>[2x]MAAAAAAEVSVDEKLDKLRAEVAKLDQISENEKAGFISLVSRYLSGEAEQIEWSKIQTPTDEVVVPYDTLASPPEDLEETKKLLDKLVVLKLNGGLGTTMGCTGPKSVIEVRNGFTFLDLIVIQIESLNKKYGCSVPLLLMNSFNTHDDTQKIVEKYSNSNIEIHTFNQSQYPRIVTEDFLPLPSKGKSGKDGWYPPGHGDVFPSLNNSGKLDILLAQGKEYVFIANSDNLGAIVDIKILNHLINNQNEYCMEVTPKTLADVKGGTLISYEGRVQLLEIAQVPDEHVNEFKSIEKFKIFNTNNLWVNLKAIKRLVEAEALKMEIIPNPKEVDGVKVLQLETAAGAAIRFFDKAIGINVPRSRFLPVKATSDLLLVQSDLYTLVDGFVIRNPARANPANPSIELGPEFKKVANFLARFKSIPSIVELDSLKVSGDVWFGSGITLKGKVTITAKSGVKLEIPDGAVLENKDVNGPEDL

UGPase is an enzyme ubiquitously distributed in all types of organisms and catalyses the formation of UDP-glucose, the key precursor of the sucrose biosynthesis and cell wall metabolism in plants. Among the various enzymes, UDP-glucose pyrophosphorylase (UGPase; EC 2.7.7.9) is important and essential in this carbon regulation, whereas the sugar, UDP-glucose, represents an important branch point in the C channel directing for synthesis of starch, sucrose or cellulose. To better comprehend the regulation and activity in the reactions involved in the saccharide metabolism, UGPases from different types of organisms have been characterized over the years. It is known that oligomerization plays a role in the regulatory process of these enzymes affecting their function and activity. Recently, the UGPase from sugarcane (ScUGPase-1) was characterized, showing that the enzymatic activity and regulatory mechanism are similar to those reported for other UGPases.

In this study, we present the first crystal structure of UGPase-1 from sugarcane at a resolution of 2.0 Å. The crystals have the symmetry of the triclinic space group P1 and diffracted to 2.0 Å resolution. The crystals of ScUGPase-1 contain two molecules per asymmetric unit, labelled monomers A and B, eight sulfate ions from the crystallization buffer, three molecules of ethylene glycol from the cryoprotectant solution and 353 water molecules. Similar to other UGPases, each monomer of ScUGPase-1 contains three domains: an N-terminal domain, a catalytic domain and a C-terminal domain. The catalytic domain consists of a mixed nine-stranded β-sheet (β1-β6, β9, β10 and β13) as a core, surrounded by six α-helices (α3-α9), and resembles a Rossmann fold. The C-terminal domain consists of 10 β-strands (β14-β23) and two α-helices (α11-α12), with the motif RFKS419IPSI, essential for the phosphorylation and binding with 14-3-3 protein, between α12 and β17. Hence, the uridinyl group is likely stabilized by Gly94, Gln169 and Gly198, whereas the glucose portion would be coordinated by Asn227, Gly265, Glu278, Asn300 and Leu92, though no electron density was observed for Gly265 in the structure of ScUGPase-1. A slight difference observed in the active site of ScUGPase-1 is the orientation of the side chain of His199. In the AtUGPase structure, the side chain is orientated closer to the β-phosphate, whereas in the ScUGPase-1 structure it is orientated closer to the α-phosphate. Analysis of ScUGPase-1 revealed a buried surface area of 480 Å2 between monomers A and B, and a complexation significance score (CSS) of 0, indicating the corresponding dimer is unlikely to be stable.Lipoprotein(a) (Lp(a)), an independent, causal cardiovascular risk factor, is a lipoprotein particle that is formed by the interaction of a low-density lipoprotein (LDL) particle and apolipoprotein(a) (apo(a)). Lp(a) is a lipoprotein particle that is formed by a two-step process involving interactions between a LDL particle and another protein, apo(a). The goal of our research was to develop a potent and selective orally delivered small-molecule therapeutic to inhibit the formation of Lp(a) by blocking the first interaction between apo(a) and apoB to reduce the circulating levels of Lp(a). In summary, we report the discovery and optimization of potent and selective small-molecule inhibitors of Lp(a) formation by exploiting the repeated KIV domain structure of apo(a) through compound multivalency.

Taking further advantage of multivalency, a trimeric molecule, LY3473329, was synthesized. Crystal structure analysis of the interactions between LY3473329 and KIV8 shows that the trimeric molecule is capable of binding to three KIV8 domains simultaneously, which suggests that multi-KIV domain interactions are possible in apo(a). LY3473329-HCl salt binds to KIV8 selectively with a potency of 22 nM and inhibits the formation of Lp(a) particles in vitro with an IC50 value of 0.09 nM (n = 9). In the Lp(a) transgenic mouse model, the plasma levels of LY3473329-HCl salt increased in a dose-dependent manner, and treatment with LY3473329-HCl reduced the levels of Lp(a) with an absolute ED50 of 3 mg kg−1, with a maximum Lp(a) reduction of 92% after five days of BID oral dosing. In cynomolgus monkeys, LY3473329 reduced median Lp(a) levels in a dose-dependent manner by up to 71% in the 100 mg kg−1 once daily (QD) cohort, compared with baseline. Multivalency, which allowed the engagement of multiple apo(a) KIV domains, considerably increased the potency and efficacy of inhibitors of Lp(a) formation in both in vitro and in vivo models of Lp(a) reduction, as compared with monovalency. A comparison of residues near the inhibitor-binding site reveals that only human PLG K-2 preserves the DxE side chains that make key interactions with LY3473329. Oral doses of prototype compounds and a potent, multivalent disruptor, LY3473329 (muvalaplin), reduced the levels of Lp(a) in transgenic mice and in cynomolgus monkeys. Although multivalent molecules bind to the Kringle domains of rat plasminogen and reduce plasmin activity, species-selective differences in plasminogen sequences suggest that inhibitor molecules will reduce the levels of Lp(a), but not those of plasminogen, in humans. These data support the clinical development of LY3473329—which is already in phase 2 studies—as a potent and specific orally administered agent for reducing the levels of Lp(a).

>APTENSTGVQDCYRGDGQSYRGTLSTTITGRTCQSWSSMTPHWHRRIPLYYPNAGLTRNYCRNPDAEIRPWCYTMDPSVRWEYCNLTRCPVTES[3x]>[8x]MAHHHHHHMNKLTLADWQHKAASLEIEGRAFIDGASRDAHGGRTFDCVSPIDGRVLAKVADCGEADVNAAVAAARRAFDAGVWAGLNPRARKAVLLRWAALMREHLDELSLLETLDAGKPIGDTTTVDVPGAAYCVEWFAEAIDKVGGEVAPADHHLVGLVTREPVGVVAAV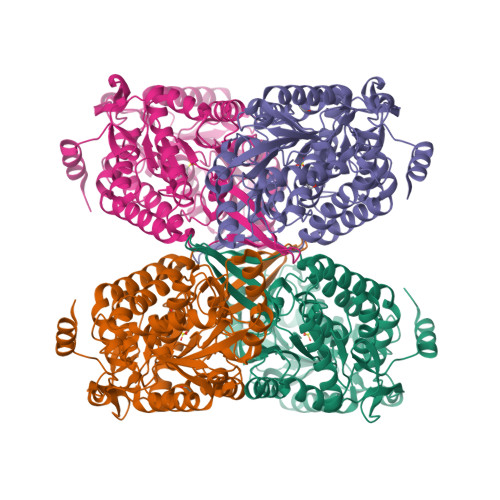VPWNFPILMAAWKFGPALAAGNSVVLKPSEKSPLTAIRVAQLAFEAGIPAGVFNVVPGAGEPGKLLALHRDVDCIAFTGSTAVGKLIMQYAAQSNLKRAWLELGGKSPNIVLPDCPDLDRAAQTAAGAIFYNMGEMCTAGSRLLVHRDIKDAFIEKLVAAARAYVPGNPLDPSVSMGAIVDGIQLERVLGYIEAGRGEGRLVTGGARVNAETGGFYVEPTVFEVKPDAKIAREEIFGPVLSVIVFDDVDEAVRIANDTEYGLAAAVWTSNLTTAHDVSRRLRAGTVWVNCYDEGGDMNFPFGGYKQSGNGRDKSLHALEKYTELKSTLIRLR> FQASPSQSLYREIHQLISFKDVLPDKNLLPDWSSNKNPCTFDGVTCRDDKVTSIDLSSKPLNVGFSAVSSSLLSLTGLESLFLSNSHINGSVSGFKCSASLTSLDLSRNSLSGPVTTLTSLGSCSGLKFLNVSSNTLDFPGKVSGGLKLNSLEVLDLSANSISGANVVGWVLSDGCGELKHLAISGNKISGDVDVSRCVNLEFLDVSSNNFSTGIPFLGDCSALQHLDISGNKLSGDFSRAISTCTELKLLNISSNQFVGPIPPLPLKSLQYLSLAENKFTGEIPDFLSGACDTLTGLDLSGNHFYGAVPPFFGSCSLLESLALSSNNFSGELPMDTLLKMRGLKV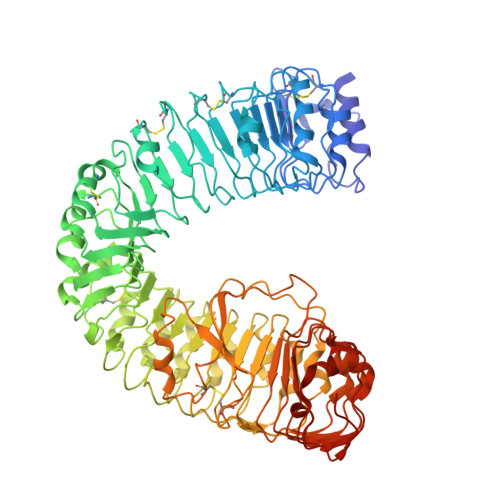LDLSFNEFSGELPESLTNLSASLLTLDLSSNNFSGPILPNLCQNPKNTLQELYLQNNGFTGKIPPTLSNCSELVSLHLSFNYLSGTIPSSLGSLSKLRDLKLWLNMLEGEIPQELMYVKTLETLILDFNDLTGEIPSGLSNCTNLNWISLSNNRLTGEIPKWIGRLENLAILKLSNNSFSGNIPAELGDCRSLIWLDLNTNLFNGTIPAAMFKQSGKIAANFIAGKRYVYIKNDGMKKECHGAGNLLEFQGIRSEQLNRLSTRNPCNITSRVYGGHTSPTFDNNGSMMFLDMSYNMLSGYIPKEIGSMPYLFILNLGHNDISGSIPDEVGDLRGLNILDLSSNKLDGRIPQAMSALTMLTEIDLSNNNLSGPIPEMGQFETFPPAKFLNNPGLCGYPLPRCDPSNADGYAHHQRSHHHHHH> MQQGQMAYDRAITVFSPDGRLFQVEYAREAVKKGSTALGMKFANGVLLISDKKVRSRLIEQNSIEKIQLIDDYVAAVTSGLV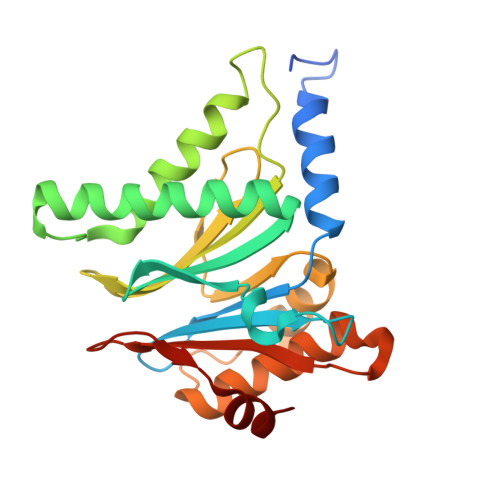ADARVLVDFARISAQQEKVTYGSLVNIENLVKRVADQMQQYTQYGGVRPYGVSLIFAGIDQIGPRLFDCDPAGTINEYKATAIGSGKDAVVSFLEREYKENLPEKEAVTLGIKALKSSLEEGEELKAPEIASITVGNKYRIYDQEEVKKFL> SMIEIDGRSLRVEDVYAVAVEYDRVSISDDTLKAVEEKHEAFLKLINSGKTVYGVNTGFGSLLNVHIERDQEIELQKNLIRSHSSGVGDYLENRYVRAIMAVRLNSLAAGYSAVSADLLNMMVEML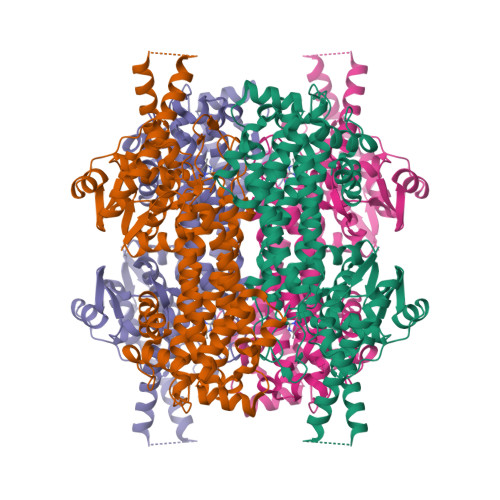NRDVIPAVPKYGSVGASGDLAPLAHIGLAMMGEGKAFFEGRLMDSARALEKAGLKPYQFKEKEGVALINGTSFMSGILSIAVMDAHDILENAIRSALLSFEALGGTSKAFTPWILGARPHLGQVAIGNRFREYLTGSDIVKRADSVKVQDAYTLRCIPQVYGSVADVIDYVENVLSVEINSATDNPLFNGEEVVSGGNFHGEPVALAADFLAIALTDLGNMVERRIARLVDTNLSGLPPFLTPDSGLNSGYMIPQYTAAALCNRNKVLAYPSSADTIPTSANQEDHVSMGATGSLKLLEIIDNVRYIIAIEYLLGSQALEFTDKGMSPSTRKIYEKIREKVEKLDHDRPPSFDIETIRKMMDKKEFISALP> MAPITFRKSYTIVPAEPTWSGRFPLAEWDQVGTITHIPTLYFYDKPSESFQGNVVEILKTSLSRVLVHFYPMAGRLRWLPRGRFELNCNAEGVEFIEAESEGKLSDFKDFSPTPEFENLMPQVNYKNPIETIPLFLAQVTKFKCGGISLSVNVSHAIVDGQSALHLISEWGRLARGEPLETVPFLDRKILWAGEPLPPFVSPPKFDHKEFDQPPFLIGETDNVEERKKKTIVVMLPLSTSQLQKLRSKANGSKHSDPAKGFTRYETVTGHVWRCACKARGHSPEQPTALGICIDTRSRMEPPLPRGYFGNATLDVVAASTSGELISNELGFAASLISKAIKNVTNEYVMIGIEYLKNQKDLKKFQDLHALGSTEGPFYGNPNLGVVSWLTLPMYGLDFGWGKEFYTGPGTHDFDGDSLILPDQNEDGSVILATCLQVAH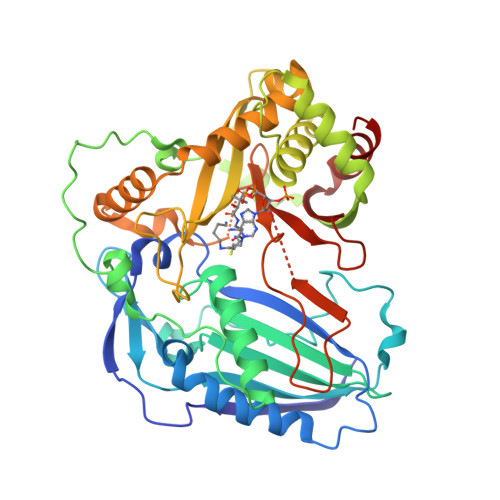MEAFKKHFYEDI>[2x]MTDVSKPSTRVTRLDEKQSTSRERLDDLLDTIPLATVALVRDGHPVAFPIGFGRVGDELVIHGSTGSPWLRALAEGAPAAVSVTALDGVVVARSS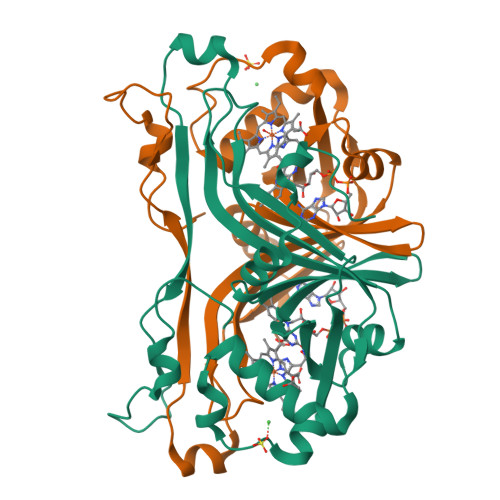FESSFRYRSATLFGTFEVIADDAKRGYLDALTDRFIPGRTAELRASTRKELAATLALALAIGDDNWSLKLSEGWPDDADEDIAAGGWAGVVPLTTQYGAPLTAPDVAAGTPLPPSVRGMTGELRNTRAR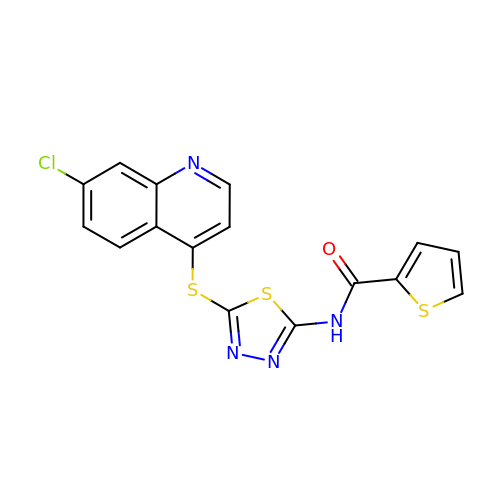N-{5-[(7-chloroquinolin-4-yl)sulfanyl]-1,3,4-thiadiazol-2-yl}thiophene-2-carboxamide | C16 H9 Cl N4 O S3 | KWDHWMGDHBBJIA-UHFFFAOYSA-N> GSDDGAFGDIWAYMSEALTGAPGKIIACG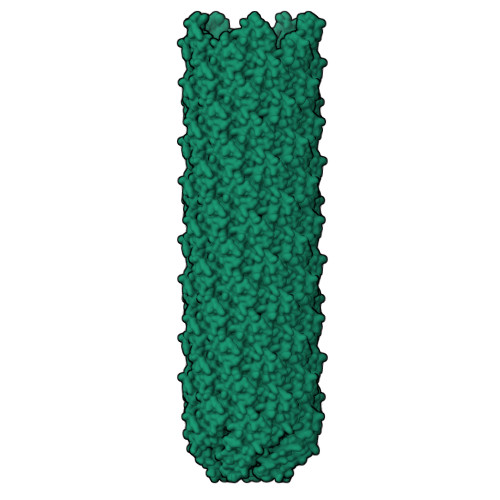MLFSVAYFGVVKPNLGLALVSALMMLVMANGEKIISSFLAAGIPL> LVAGLTPIEANGYLDFFIDRPLGMKGYILNLTIRGQGVVKNQGREFVCRPGDILLFPPGEIHHYGRHPEAREWYHQWVYFRPRAYWHEWLNWPSIFANTGFFRPDEAHQPHFSDLFGQIINAGQGEGRYSELLAINLLEQLLLRRME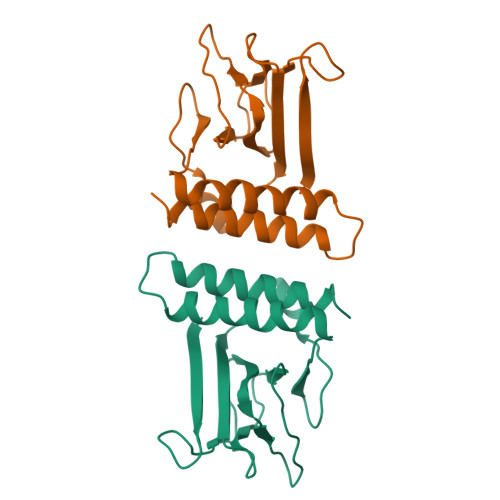AI Tc toxins consist of three components: TcA, TcB, and TcC. We therefore chose TcdB2-TccC3 to function as a cocoon scaffold for translocation of other cargo proteins, which are not components of the Tc toxin system.

In case of the wild-type TccC3HVR, the affinity of TcB-TcC to TcA is in the picomolar range, resulting in almost complete holotoxin formation. This was also the case for holotoxins composed of TcA and cocoons containing Cdc42 (20.3 kDa) and TEV (28.1 kDa). TEV protease is not an exceptionally stable protein, as it unfolds at ~ 52 °C38. However, it contains two small β-barrels, which are known to be a notoriously stable fold. Therefore, we believe that these domains are more rigid than the native Tcc3HVR or other translocated cargos such as HVR128-iLOV, which might prevent the protein from being translocated. To prove this, we determined the structure of TcB-TcC-TEV to a resolution of 3.7 Å using X-ray crystallography. The cocoon of TcB-TcC-TEV shows an identical size and shape to the TcB-TcC(WT) cocoon, with a Cα RMSD of 0.552 Å2. However, the electron density inside appears already at a higher sigma level, indicating that the encapsulated TEV is indeed more rigid and ordered than the native TccC3HVR. This is the likely cause for TEV not being translocated. As folded proteins do not fit through the narrow constriction site of the translocation channel, the formation of defined structural elements such as β-barrels in the cocoon probably results in translocation arrest. Therefore, a third prerequisite needs to be fulfilled: the encapsulated cargo must not form any tertiary structures or stably interact with the cocoon. The two abovementioned cargos violate this prerequisite, with TEV containing two highly stable β-barrels, and Cdc42 possessing an amphipathic C-terminus that associates with a hydrophobic binding pocket in the cocoon.

> MQNSQDFSITELSLPKGGGAITGMGEALTPTGPDGMAALSLPLPISAGRGYAPAFTLNYNSGAGNSPFGLGWDCNVMTIRRRTHFGVPHYDETDTFLGPEGEVLVVADQPRDESTLQGINLGATFTVTGYRSRLESHFSRLEYWQPKTTGKTDFWLIYSPDGQVHLLGKSPQARISNPSQTTQTAQWLLEASVSSRGEQIYYQYRAEDDTGCEADEITHHLQATAQRYLHIVYYGNRTASETLPGLDGSAPSQADWLFYLVFDYGERSNNLKTPPAFSTTGSWLCRQDRFSRYEYGFEIRTRRLCRQVLMYHHLQALDSKITEHNGPTLVSRLILNYDESAIASTLVFVRRVGHEQDGNVVTLPPLELAYQDFSPRHHAHWQPMDVLANFNAIQRWQLVDLKGEGLPGLLYQDKGAWWYRSAQRLGEIGSDAVTWEKMQPLSVIPSLQSNASLVDINGDGQLDWVITGPGLRGYHSQRPDGSWTRFTPLNALPVEYTHPRAQLADLMGAGLSDLVLIGPKSVRLYANTRDGFAKGKDVVQSGDITLPVPGADPRKLVAFSDVLGSGQAHLVEVSATKVTCWPNLGRGRFGQPITLPGFSQPATEFNPAQVYLADLDGSGPTDLIYVHTNRLDIFLNKSGNGFAEPVTLRFPEGLRFDHTCQLQMADVQGLGVASLILSVPHMSPHHWRCDLTNMKPWLLNEMNNNMGVHHTLRYRSSSQFWLDEKAAALTTGQTPVCYLPFPIHTLWQTETEDEISGNKLVTTLRYARGAWDGREREFRGFGYVEQTDSHQLAQGNAPERTPPALTKNWYATGLPVIDNALSTEYWRDDQAFAGFSPRFTTWQDNKDVPLTPEDDNSRYWFNRALKGQLLRSELYGLDDSTNKHVPYTVTEFRSQVRRLQHTDSRYPVLWSSVVESRNYHYERIASDPQCSQNITLSSDRFGQPLKQLSVQYPRRQQPAINLYPDTLPDKLLANSYDDQQRQLRLTYQQSSWHHLTNNTVRVLGLPDSTRSDIFTYGAENVPAGGLNLELLSDKNSLIADDKPREYLGQQKTAYTDGQNTTPLQTPTRQALIAFTETTVFNQSTLSAFNGSIPSDKLSTTLEQAGYQQTNYLFPRTGEDKVWVAHHGYTDYGTAAQFWRPQKQSNTQLTGKITLIWDANYCVVVQTRDAAGLTTSAKYDWRFLTPVQLTDINDNQHLITLDALGRPITLRFWGTENGKMTGYSSPEKASFSPPSDVNAAIELKKPLPVAQCQVYAPESWMPVLSQKTFNRLAEQDWQKLYNARIITEDGRICTLAYRRWVQSQKAIPQLISLLNNGPRLPPHSLTLTTDRYDHDPEQQIRQQVVFSDGFGRLLQAAARHEAGMARQRNEDGSLIINVQHTENRWAVTGRTEYDNKGQPIRTYQPYFLNDWRYVSNDSARQEKEAYADTHVYDPIGREIKVITAKGWFRRTLFTPWFTVNEDENDTAAEVKKVKMPGSRPMKNIDPKLYQKTPTVSVYDNRGLIIRNIDFHRTTANGDPDTRITRHQYDIHGHLNQSIDPRLYEAKQTNNTIKPNFLWQYDLTGNPLCTESIDAGRTVTLNDIEGRPLLTVTATGVIQTRQYETSSLPGRLLSVAEQTPEEKTSRITERLIWAGNTEAEKDHNLAGQCVRHYDTAGVTRLESLSLTGTVLSQSSQLLIDTQEANWTGDNETVWQNMLADDIYTTLSTFDATGALLTQTDAKGNIQRLAYDVAGQLNGSWLTLKGQTEQVIIKSLTYSAAGQKLREEHGNDVITEYSYEPETQRLIGIKTRRPSDTKVLQDLRYEYDPVGNVISIRNDAEATRFWHNQKVMPENTYTYDSLYQLISATGREMANIGQQSHQFPSPALPSDNNTYTNYTRTYTYDRGGNLTKIQHSSPATQNNYTTNITVSNRSNRAVLSTLTEDPAQVDALFDAGGHQNTLISGQNLNWNTRGELQQVTLVKRDKGANDDREWYRYSGDGRRMLKINEQQASNNAQTQRVTYLPNLELRLTQNSTATTEDLQVITVGEAGRAQVRVLHWESGKPEDIDNNQLRYSYDNLIGSSQLELDSEGQIISEEEYYPYGGTALWAARNQTEASYKTIRYSGKERDATGLYYYGYRYYQPWIGRWLSSDPAGTIDGLNLYRMVRNNPVTLLDPDGLMPEFGESLFKGPRDYNPISSTICHLTNESDGHTTSLYGIGFGPFIITNKHLFRRNNGTLLVQSLHGVFKVKNTTTLQQHLIDGRDMIIIRMPKDFPPFPQKLKFREPQREERICLVTTNFQTKSMSSMVSDTSCTFPSSDGIFWKHWIQTKDGQCGSPLVSTRDGFIVGIHSASNFTNTNNYFTSVPKNFMELLTNQEAQQWVSGWRLNADSVLWGGHKVFMVKPEEPFQPVKEATQLMNRRRRRLEHHHHHH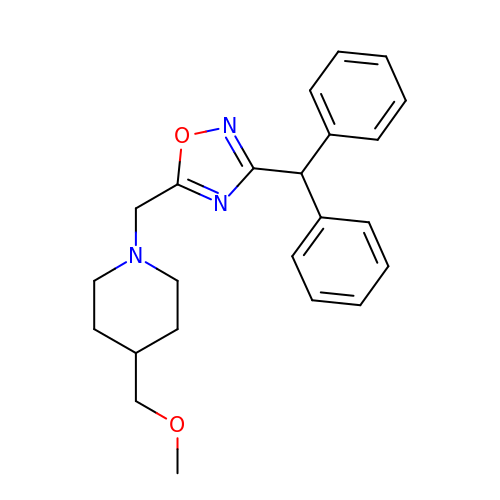1-{[3-(diphenylmethyl)-1,2,4-oxadiazol-5-yl]methyl}-4-(methoxymethyl)piperidine | C23 H27 N3 O2 | XYPQCOBQQQTCFN-UHFFFAOYSA-N> QPCPGRCICQNVAPTLTMLCAKTGLLFVPPAIDRRVVELRLTDNFIAAVRRRDFANMTSLVHLTLSRNTIGQVAAGAFADLRALRALHLDSNRLAEVRGDQLRGLGNLRHLILGNNQIRKVESAAFDAFLSTVEDLDLSYNNLEALPWEAVGQMVNLNTLTLDHNLIDHIAEGTFVQLHKLVRLDMTSNRLHKLPPDGLFLRSQGGGPKPPTPLTVSFGGNPLHCNCELLWLRRLTREDDLETCATPEHLTDRYFWSIPEEEFLCEPP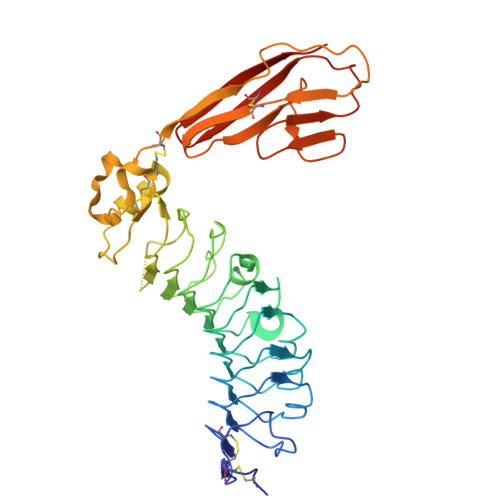LITRQAGGRALVVEGQAVSLRCRAVGDPEPVVHWVAPDGRLLGNSSRTRVRGDGTLDVTITTLRDSGTFTCIASNAAGEATAPVEVCVVPLHHHHHH> GSRLETEIERCRSECQWERIPELVKQLSAKLIANDDMAELLLGESKLEQYLKEHPLRQGASPRGPKPQLTEVRKHLTAALDRGNLKSEFLQESNLIMAKLNYVEGDYKEALNIYARVGLDDLPLTAVPPYRLRVIAEAYATKGLCLEKLPISSSTSNLHVDREQDVITCYEKAGDIALLYLQEIERVILSNIQNRSPKPGPAPHDQELGFFLETGLQRAHVLYFKNGNLTRGVGRFRELLRAVETRTTQNLRMTIARQLAEILLRGMCEQSYWNPLEDPPCQSPLDDPLRKGANTKTYTLTRRARVYSGENIFCPQENTEEALLLLLISESMANRDAVLSRIPEHKSDRLISLQ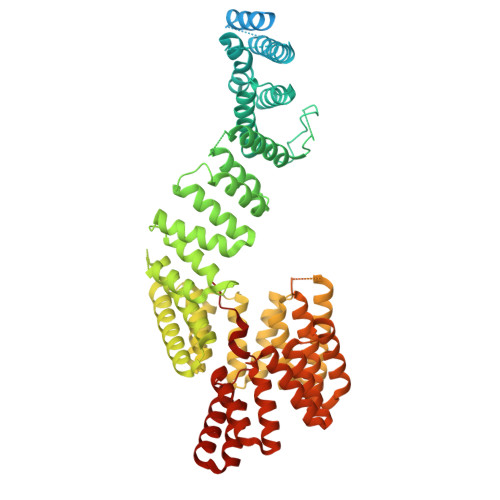SASVVYDLLTIALGRRGQYEMLSECLERAMKFAFEEFHLWYQFALSLMAAGKSARAVKVLKECIRLKPDDATIPLLAAKLCMGSLHWLEEAEKFAKTVVDVGEKTSEFKAKGYLALGLTYSLQATDASLRGMQEVLQRKALLAFQRAHSLSPTDHQAAFYLALQLAISRQIPEALGYVRQALQLQGDDANSLHLLALLLSAQKHYHDALNIIDMALSEYPENFILLFSKVKLQSLCRGPDEALLTCKHMLQIWKSCYNLTNPSDSGRGSSLLDRTIADRRQLNTITLPDFSDPETGSVHATSVAASRVEQALSEVASSLQSSAPKQGPLHPWMTLAQIWLHAAEVYIGIGKPAEATACTQEAANLFPMSHNVLYMRGQIAELRGSMDEARRWYEEALAISPTHVKSMQRLALILHQLGRYSLAEKILRDAVQVNSTAHEVWNGLGEVLQAQGNDAAATECFLTALELEASSPAVPFTIIPRVL>[2x]G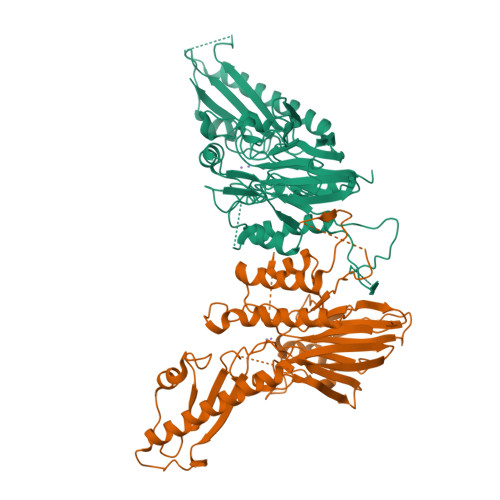PLGSENTIRILISSDPHVGYGEKDPVRGNDSFVSFNEILEIARERDVDMILLGGDIFHDNKPSRKALYQALRSLRLNCLGDKPCELELLSDTSLTTGDTAVCNINYLDPNINVAIPVFSIHGNHDDPSGDGRYSALDILQVTGLVNYFGRVPENDNIVVSPILLQKGFTKLALYGISNVRDERLYHSFRENKVKFLRPDLYRDEWFNLLTVHQNHSAHTPTSYLPESFIQDFYDFVLWGHEHECLIDGSYNPTQKFTVVQPGSTIATSLSPGETAPKHCGILNITGKDFHLEKIRLRTVRPFIMKDIILSEVSSIPPMVENKKEVLTYLISKVEEAITEANAQWYEAQGTVPVVENEKPPLPLIRLRVDYTGGYQTENPQRFSNRFVGRVANATDVVQFYLKK> MANNSF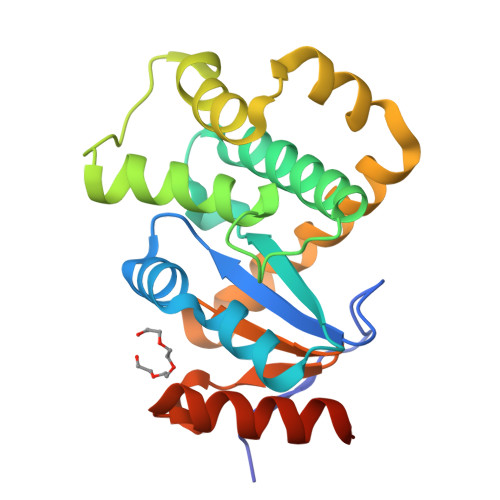ITLNPSLPNSENSVIEAFSYKCIHCYNHHKFGTLEKLREAFPNLHFKLYPVSLMNGEFSKEMNELFAFAQYKDEQNGKDASYSDSLSHKLADVYFVSYFLNKQRNFSNLDEFYDIGLKAMNVNKNEVLNFLNTPKAKEILSEFQRANDIAKTYGTPAFVVNGKYQINPSAINSMQDLEDLVKKLSNMKLEHHHHHH> MTENRYFFAIRYLSDD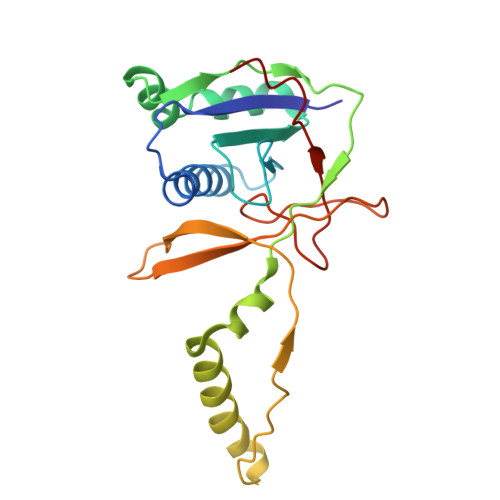VDCGLLAGRCISILHGFRQAHPGIQIGVAFPEWSDRDLGRSIAFVSTNKSLLERFRERSYFQVMQADNFFALSLVLEVPDTCQNVRFIRNQNLAKLFVGERRRRLARAKRRAKARGEAFQPHMPDETKVVGVFHSVFMQSASSGQSYILHIQKHRYERSEDSGYSSYGLASNDLYTGYVPDLGAIFSTLF> PNYCFAGKTSSISDLKEVPRKNITLIRGLGHGAFGEVYEGQVSGMPNDPSPLQVAVKTLPEVCSEQDELDFLMEALIISKFNHQNIVRCIGVSLQSLPRFILLELMAGGDLKSFLRETRPRPSQPSSLAMLDLLHVARDIA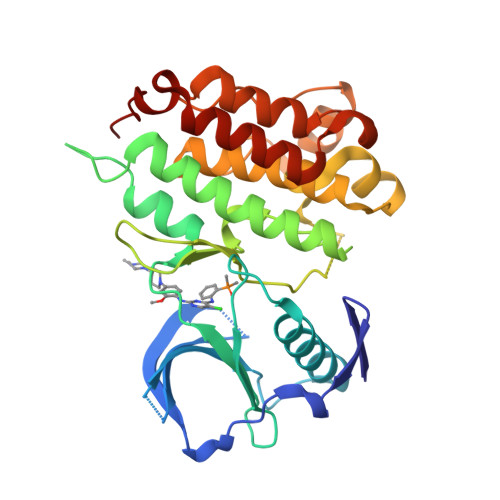CGCQYLEENHFIHRDIAARNCLLTCPGPGRVAKIGDFGMARDIYRASYYRKGGCAMLPVKWMPPEAFMEGIFTSKTDTWSFGVLLWEIFSLGYMPYPSKSNQEVLEFVTSGGRMDPPKNCPGPVYRIMTQCWQHQPEDRPNFAIILERIEYCTQDPDVINTALPIE> UCG;> CCCUCU;> GGUUUGGAGGGAAAAGUUAUCAGGCAUGCACCUGGUAGCUAGUCUUUAAACCAAUAGAUUGCAUCGGUUUAAAAGGCAAGACCGUCAAAUUGCGGGAAAGGGGUCAACAGCCGUUCAGUACCAAGUCUCAGGGGAAACUUUGAGAUGGCCUUGCAAAGGGUAUGGUAAUAAGCUGACGGACAUGGUCCUAACCACGCAGCCAAGUCCUAAGUCAACAGAUCUUCUGUUGAUAUGGAUGCAGUUCACAGACUAAAUGUCGGUCGGGGAAGAUGUAUUCUUCUCAUAAGAUAUAGUCGGACCUCUCCUUAAUGGGAGCUAGCGGAUGAAGUGAUGCAACACUGGAGCCGCUGGGAACUAAUUUGUAUGCGAAAGUAUAUUGAUUAGUUUUGGAGU

Group I introns catalyze their own excision from RNA precursors in many organisms through two sequential transesterification reactions. The Tetrahymena thermophila group I self-splicing intron was the first ribozyme to be discovered. To understand how the group I intron promotes catalysis and coordinates self-splicing reactions, we determine the structures of L-16 Tetrahymena ribozyme in complex with a 5′-splice site analog product and a 3′-splice site analog substrate using cryo-EM.

We captured two additional states (Con5-6) that may represent a substrate release process. There are high cross-correlation coefficients among Con4-6 maps (CC = 0.98). At the nucleotide level, the major difference lies in the 5′-end of the intron, with negligible changes in the catalytic core. In Con5, only the first few base pairs of the P1-P10 duplex can be observed, which is even worse in Con6, indicating a possibility that an unpairing process has been ongoing in the P1-P10 duplex. The fact that undocked P1-P10 is stacked in continuity of P2 after ligation and start to unpair from P10 suggests that the contact between P2.1 and undocked P1-P10 might favor strand dissociation for freeing the ligated exons. Finally, the 5′-exon loses tertiary interactions with the intron and the exon product becomes undocked, followed by duplex unpairing to release the product (Con4-6).>GSHMTHPTHPAAALEPIETASRDELQALQLERLKWSLRHAYDNVPHYRRTFDAAGVHPDDLKSLADLAKFPFSTKNDLRDNYPFGLFAVPREQVVRVHASSGTTGKPTVVGYTARDIDTWANVTARSIRAAGGRPGDTLHNAFGYGLFTGGLGIHYGAERLGCMVVPMSGGQTEKQVQLIRDFEPKIILVTPSYMLNLIDEMVRQGMDPAESSLKIGIFGAEPWTQALRNEVETRVGIDALDIYGLSEVMGPGVACECVETKDGPVIWEDHFYPEIIDPVTGEVLPDGSQGELVFTSLTKEAMPVIRYRTRDLTALLPPTARAMRRLAKITGRSDDMLIVRGVNVFPSQIEEIVVALPLLSGQFQI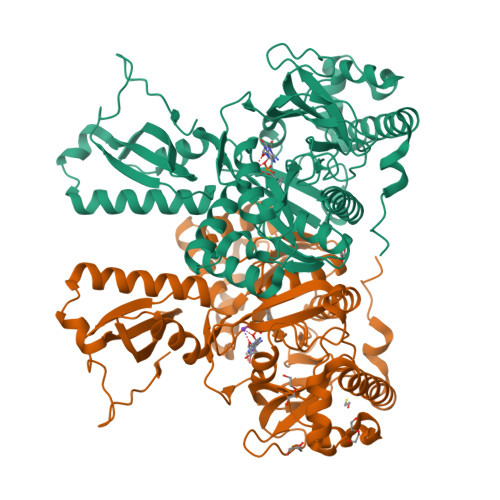TLSRDGHMDRLDLAVELRSEAAASVTDGERAALARELQHRIKTMVGVSSGVTVLAAGGIPATATGKARRVIDRRQAA[2x]> MGRKKFEAFGFVCLISLLLLFNSLWLASSNMEGDALHSLRANLVDPNNVLQSWDPTLVNPCTWFHVTCNNENSVIRVDLGNADLSGQLVPQLGQLKNLQYLELYSNNITGPVPSDLGNLTNLVSLDLYLNSFTGPIPDSLGKLFKLRFLRLNNNSLTGPIPMSLTNIMT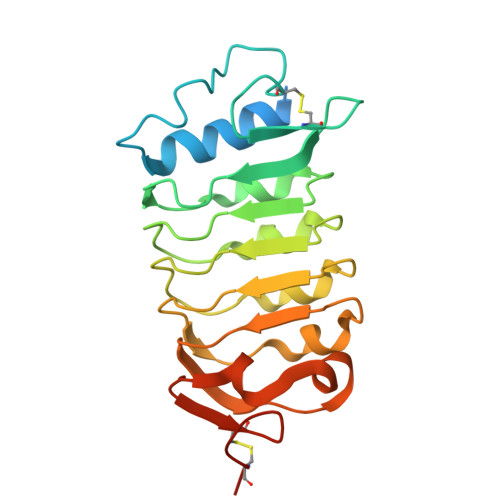LQVLDLSNNRLSGSVPDNGSFSLFTPISFANNLDLCGPVTSRPCPGSHHHHHH> MAFWTQLMLLLWKNFMYRRRQPVQLLVELLWPLFLFFILVAVRHSHPPLEHHECHFPNKPLPSAGTVPWLQGLICNVNNTCFPQLTPGEEPGRLSNFNDSLVSRLLADARTVLGGASAHRTLAGLGKLIATLRAARSTAQPQPTKQSPLEPPMLDVAELLTSLLRTESLGLALGQAQEPLH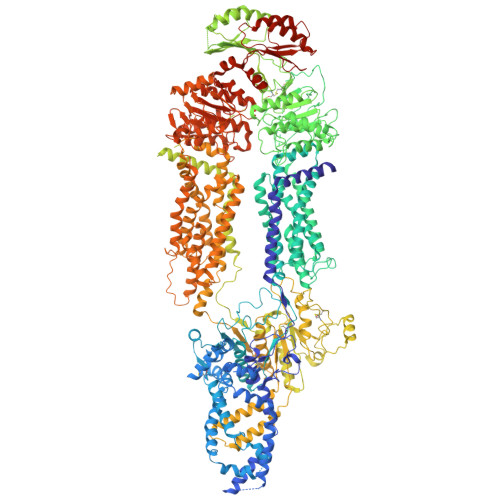SLLEAAEDLAQELLALRSLVELRALLQRPRGTSGPLELLSEALCSVRGPSSTVGPSLNWYEASDLMELVGQEPESALPDSSLSPACSELIGALDSHPLSRLLWRRLKPLILGKLLFAPDTPFTRKLMAQVNRTFEELTLLRDVREVWEMLGPRIFTFMNDSSNVAMLQRLLQMQDEGRRQPRPGGRDHMEALRSFLDPGSGGYSWQDAHADVGHLVGTLGRVTECLSLDKLEAAPSEAALVSRALQLLAEHRFWAGVVFLGPEDSSDPTEHPTPDLGPGHVRIKIRMDIDVVTRTNKIRDRFWDPGPAADPLTDLRYVWGGFVYLQDLVERAAVRVLSGANPRAGLYLQQMPYPCYVDDVFLRVLSRSLPLFLTLAWIYSVTLTVKAVVREKETRLRDTMRAMGLSRAVLWLGWFLSCLGPFLLSAALLVLVLKLGDILPYSHPGVVFLFLAAFAVATVTQSFLLSAFFSRANLAAACGGLAYFSLYLPYVLCVAWRDRLPAGGRVAASLLSPVAFGFGCESLALLEEQGEGAQWHNVGTRPTADVFSLAQVSGLLLLDAALYGLATWYLEAVCPGQYGIPEPWNFPFRRSYWCGPRPPKSPAPCPTPLDPKVLVEEAPPGLSPGVSVRSLEKRFPGSPQPALRGLSLDFYQGHITAFLGHNGAGKTTTLSILSGLFPPSGGSAFILGHDVRSSMAAIRPHLGVCPQYNVLFDMLTVDEHVWFYGRLKGLSAAVVGPEQDRLLQDVGLVSKQSVQTRHLSGGMQRKLSVAIAFVGGSQVVILDQPTAGVDPASRRGIWELLLKYREGRTLILSTHHLDEAELLGDRVAVVAGGRLCCCGSPLFLRRHLGSGYYLTLVKARLPLTTNEKADTDMEGSVDTRQEKKNGSQGSRVGTPQLLALVQHWVPGARLVEELPHELVLVLPYTGAHDGSFATLFRELDTRLAELRLTGYGISDTSLEEIFLKVVEECAADTDMEDGSCGQHLCTGIAGLDVTLRLKMPPQETALENGEPAGSAPETDQGSGPDAVGRVQGWALTRQQLQALLLKRFLLARRSRRGLFAQIVLPALFVGLALVFSLIVPPFGHYPALRLSPTMYGAQVSFFSEDAPGDPGRARLLEALLQEAGLEEPPVQHSSHRFSAPEVPAEVAKVLASGNWTPESPSPACQCSRPGARRLLPDCPAAAGGPPPPQAVTGSGEVVQNLTGRNLSDFLVKTYPRLVRQGLKTKKWVNEVRYGGFSLGGRDPGLPSGQELGRSVEELWALLSPLPGGALDRVLKNLTAWAHSLDAQDSLKIWFNNKGWHSMVAFVNRASNAILRAHLPPGPARHAHSITTLNHPLNLTKEQLSEGALMASSVDVLVSICVVFAMSFVPASFTLVLIEERVTRAKHLQLMGGLSPTLYWLGNFLWDMCNYLVPACIVVLIFLAFQQRAYVAPANLPALLLLLLLYGWSITPLMYPASFFFSVPSTAYVVLTCINLFIGINGSMATFVLELFSDQKLQEVSRILKQVFLIFPHFCLGRGLIDMVRNQAMADAFERLGDRQFQSPLRWEVVGKNLLAMVIQGPLFLLFTLLLQHRSQLLPQPRVRSLPLLGEEDEDVARERERVVQGATQGDVLVLRNLTKVYRGQRMPAVDRLCLGIPPGECFGLLGVNGAGKTSTFRMVTGDTLASRGEAVLAGHSVAREPSAAHLSMGYCPQSDAIFELLTGREHLELLARLRGVPEAQVAQTAGSGLARLGLSWYADRPAGTYSGGNKRKLATALALVGDPAVVFLDQPTTGMDPSARRFLWNSLLAVVREGRSVMLTSHSMEECEALCSRLAIMVNGRFRCLGSPQHLKGRFAAGHTLTLRVPAARSQPAAAFVAAEFPGAELREAHGGRLRFQLPPGGRCALARVFGELAVHGAEHGVEDFSVSQTMLEEVFLYFSKDQGKDEDTEEQKEAGVGVDPAPGLQHPKRVSQFLDDPSTAETVL> MWKRSEQMKIKSGKCNMAAAMETEQLGVEIFETADCEENIESQDRPKLEPFYVERYSWSQLKKLLADTRKYHGYMMAKAPHDFMFVKRNDPDGPHSDRIYYLAMSGENRENTLFYSEIPKTINRAAVLMLSWKPLLDLFQATLDYGMYSREEELLRERKRIGTVGIASYDYHQGSGTFLFQAGSGIYHVKDGGPQGFTQQPLRPNLVETSCPNIRMDPKLCPADPDWIAFIHSNDIWISNIVTREERRLTYVHNELANMEEDARSAGVATFVLQEEFDRYSGYWWCPKAETTPSGGKILRILYEENDESEVEIIHVTSPMLETRRADSFRYPKTGTANPKVTFKMSEIMIDAEGRIIDVIDKELIQPFEILFEGVEYIARAGWTPEGKYAWSILLDRSQTRLQIVLISPELFIPVEDDVMERQRLIESVPDSVTPLIIYEETTDIWINIHDIFHVFPQSHEEEIEFIFASECKTGFRHLYKITSILKESKYKRSSGGLPAPSDFKCPIKEEIAITSGEWEVLGRHGSNIQVDEVRRLVYFEGTKDSPLEHHLYVVSYVNPGEVTRLTDRGYSHSCCISQHCDFFISKYSNQKNPHCVSLYKLSSPEDDPTCKTKEFWATILDSAGPLPDYTPPEIFSFESTTGFTLYGMLYKPHDLQPGKKYPTVLFIYGGPQVQLVNNRFKGVKYFRLNTLASLGYVVVVIDNRGSCHRGLKFEGAFKYKMGQIEIDDQVEGLQYLASRYDFIDLDRVGIHGWSYGGYLSLMALMQRSDIFRVAIAGAPVTLWIFYDTGYTERY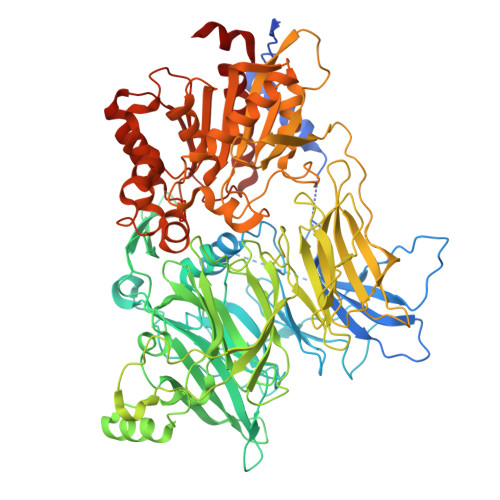MGHPDQNEQGYYLGSVAMQAEKFPSEPNRLLLLHGFLDENVHFAHTSILLSFLVRAGKPYDLQIYPQERHSIRVPESGEHYELHLLHYLQENLGSRIAALKVI> VRLPGLAAMRQGTRLFTPEQGEDLREALRRRRGSFQTTCEVTSETTFAAARRLREKASALAALNFASAKNPGGGFLGGAQAQEEDLCRGSGLYFSLTSPQAEPYYAVNRQSHSALYTDHLIYSPQVPIFRDDAGQLLPAPVPVNIITAPAPNAGAVAQSRPEQLPQVLPTLRERARRVLGVAAWMEQTHLVLGAWGCGVFRNDPAGVARTFRELLEGEAQGAFEHVTFAVLDNHPQHPKLGAFRRELESLC

Despite the abundance of PARP1, most of the PAR generated by DNA damage is rapidly degraded, with a half-life of less than 1 min by poly (ADP-ribose) glycohydrolase (PARG). The radio-resistant bacterium D. radiodurans encodes a PARG homolog, DrPARG, whose expression is upregulated after radiation damage, so it might play an important role in DNA repair. Our study demonstrates that DrPARG is involved in catalyzing the breakdown of endogenous PAR and DNA repair in D. radiodurans. From observing the structural peculiarities of DrPARG, we show that although previously thought to be an obligate exo-glycohydrolase, bacterial PARG could exert both exo- and endo-glycohydrolase functions.

To clarify the effect of Thr267 on enzyme activity of DrPARG, we generated mutants of DrPARG by substituting Thr267 for arginine or lysine. Furthermore, we determined crystal structures of DrPARG T267R and T267K in complex with ADP-ribose for understanding the detailed interactions. The crystal structures of T267R and T267K belonged to the space group P3221. In consistent to the secondary structure analyzed by CD spectrum, the substitution of the residue did not cause dramatic alterations to overall structure compared with the wild-type enzyme with root mean square deviation to wild type of 0.50 and 0.43 Å for T267R and T267K, respectively. The side chain of Lys267 did not form hydrogen bonding with neighboring residues, but positioned toward the side chain of Asp260 by ionic interaction. The superposition of the modeled PAR trimer and the DrPARG T267K structure showed that the n + 1 unit was blocked by the barrier resulted from ionic pairing of side chains of Lys267 and Asp260 and implicated that the ionic bonding might be sufficient for establishing the steric hindrance of the exo-glycohydrolase mode. Compared with the solvent-accessible 2′-OH with n + 1 linkage point observed in wild-type, which were inaccessible and less accessible to solvent in the complex structures of T267R and T267K, respectively. PARG cleavage assay in vitro showed T267R and T267K mutants with decreased hydrolysis PAR activity as compared with the wild-type enzyme. Short-chain PAR was not detected in the filtrates of the two DrPARG mutants T267R and T267K, as well as the TcPARG, although the mutants still hydrolyzed PAR. Since T267R and T267K DrPARG catalyze the hydrolysis of PAR without generating short-chain PAR but oligo ADP-ribose, the establishment of endo-glycohydrolase activity was not solely accounted from the lack of steric hinderance near 2′-OH.> PEASFQVWNKDSSSKNLIPRLQKIWKNYLSMNKYKVSYKGPGPGIKFSAEALRCHLRDHVNVSMVEVTDFPFNTSEWEGYLPKESIRTKAGPWGRCAV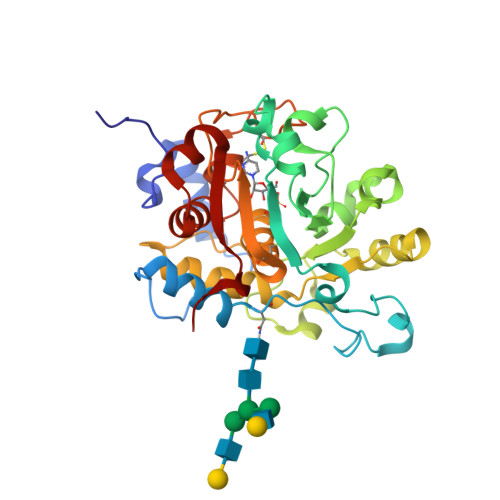VSSAGSLKSSQLGREIDDHDAVLRFNGAPTANFQQDVGTKTTIRLMNSQLVTTEKRFLKDSLYNEGILIVWDPSVYHSDIPKWYQNPDYNFFNNYKTYRKLHPNQPFYILKPQMPWELWDILQEISPEEIQPNPPSSGMLGIIIMMTLCDQVDIYEFLPSKRKTDVCYYYQKFFDSACTMGAYHPLLYEKNLVKHLNQGTDEDIYLLGKATLPGFRTIHC> SNAMNERSRPLRFDSLTQEAYLQLWRTYDRMKAIEEEIFSQFELSAQQYNTLRLLRSVHPEGMATLQIADR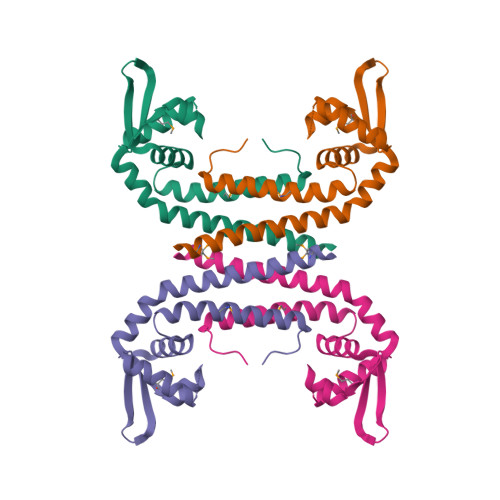LISRAPDITRLIDRLDDRGLVLRTRKPENRRVVEVALTDAGLKLLKDLEEPVRQCHERQLGHLAADELHELIRLMELARTPHEEPGSRWIADRSRPS> MHHHHHHNRQQIDALVKQMNVDTAKGPVDERIQQVVVRLLGDLFQAIEDLDIQPSEVWKGLEYLTDAG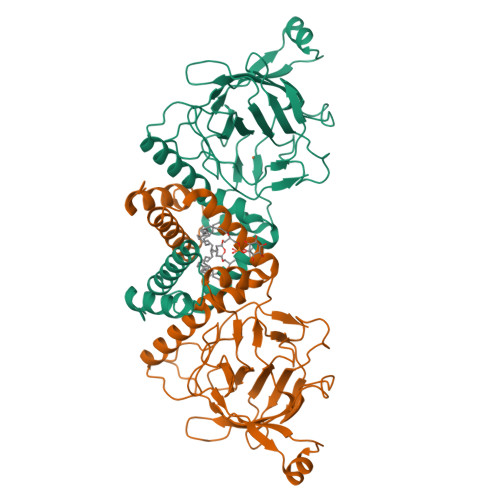QANELGALAAGLGLEHYLDLRADEADAKAGITGGTPRTIEGPLYVAGAPESVGFARMDDGSESDKVDTLIIEGTVTDTEGNIIEGAKVEVWHANSLGNYSFFDKSQSDFNLRRTILTDVNGKYVALTTMPVGYGCPPEGTTQALLNKLGRHGNRPSHVHYFVSAPGYRKLTTQFNIEGDEYLWDDFAFATRDGLVATATDVTDEAEIARRELDKPFKHITFNVELVKEAEAAPSSEVERRRASA>GHMSKSDYIQNMFQTKSFVDRYKYTEKLTGLYAQTLVDYSGVANTSQKPLIVLDNACGIGAVSSVLNHTLQDEAKKTWKLTCGDLSEGMLETTKRRLQDEGWVNAETKIVNALDTGLPDGHYTHVFVAFGFQSFPDANAALKECFRILASGGILASSTWQNFNWIPIMKAAIETIPGNLPFPTQKEFIALHNAGWDSESYIQSELEKLGFRDVKVIPVPKETSIPIDEFFEVCMMIIPYLLPKFWTEEQRESHEKDVPMVLRQYLQDTYGANGQVPLEAVALITTG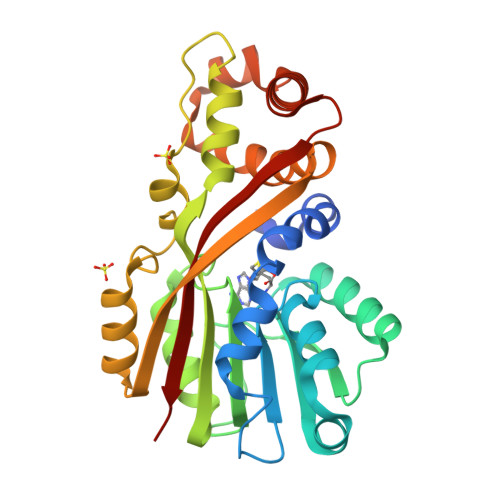LKP[2x]>[2x]MVMKHLSLTPELYKYLLDISLREHPAL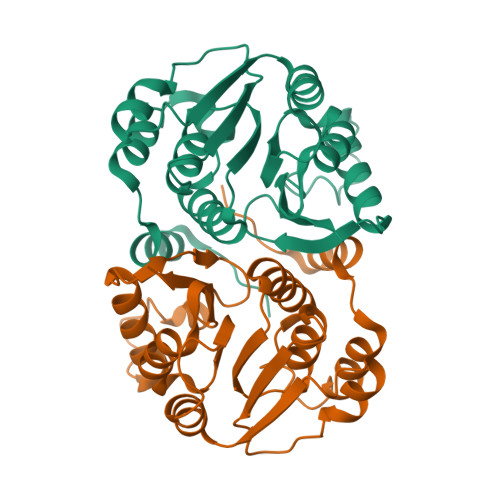AALRKETSTMELANMQVAPEQAQFMQMLIRLTRAKKVLELGTFTGYSALAMSLALPDDGQVITCDINEGWTKHAHPYWREAKQEHKIKLRLGPALDTLHSLLNEGGEHQFDFIFIDADKTNYLNYYELALKLVTPKGLIAIDNIFWDGKVIDPNDTSGQTREIKKLNQVIKNDSRVFVSLLAIADGMFLVQPIAENLYFQSHHHHHHWSHPQFEK>SMQGPRTRARLGANEVLLVVGGFGSQQSPIDVVEKYDPKTQEWSFLPSITRKRRYVASVSLHDRIYVIGGYDGRSRLSSVECLDYTADEDGVWYSVAPMNVRRGLAGATTLGDMIYVSGGFDGSRRHTSMERYDPNIDQWSMLGDMQTAREGAGLVVASGVIYCLGGYDGLNILNSVEKYDPHT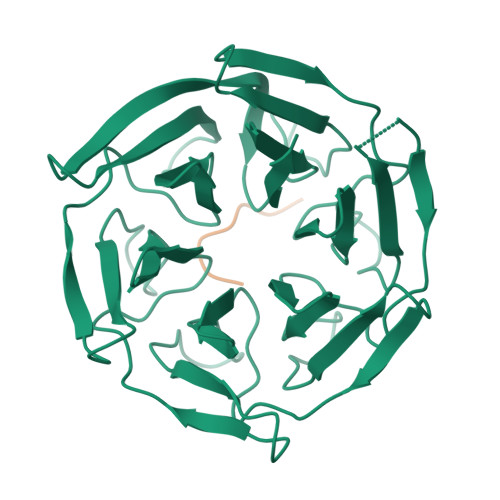GHWTNVTPMATKRSGAGVALLNDHIYVVGGFDGTAHLSSVEAYNIRTDSWTTVTSMTTPRCYVGATVLRGRLYAIAGYDGNSLLSSIECYDPIIDSWEVVTSMGTQRCDAGVCVLRE[2x];>[2x]PGAPPGRDLA>[2x]MPSEEEEKRRAKQVAKEKILEQNPSSKVQVRRVQKQGNTIRVELEITE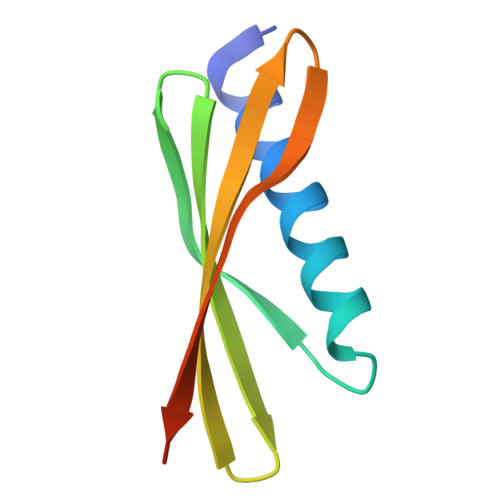NGKKTNITVEVEKQGNTFTVKRITETVGSLEHHHHHH> MAQALLVPPGPESFRLFTRESLAAIEKRAAEEKAKKPKKEQDNDDENKPKPNSDLEAGKNLPFIYGDIPPEMVSEPLEDLDPYYINKKTFIVMNKGKAIFRFSATSALYILTPLNPVRKIAIKILVHSLFSMLIMCTILTNCVFMTLSNPPDWTKNVEYTFTGIYTFESLIKILARGFCLEDFTFLRDPWNWLDFSVIVMAYVTEFVSLGNVSALRTFRVLRALKTISVIPGLKTIVGALIQSVKKLSDVMILTVFCLSVFALIGLQLFMGNLRNKCLQWPPSDSAFETNTTSYFNGTMDSNGTFVNVTMSTFNWKDYIGDDSHFYVLDGQKDPLLCGNGSDAGQCPEGYICVKAGRNPNYGYTSFDTFSWAFLSLFRLMTQDYWENLYQLTLRAAGKTYMIFFVLVIFLGSFYLVNLILAVVAMAYEEQNQATLEEAEQKEAEFQQMLEQLKKQQEEAQAVAAASAASRDFSGIGGLGELLESSSEASKLSSKSAKEWRNRRKKRRQREHLEGNNKGERDSFPKSESEDSVKRSSFLFSMDGNRLTSDKKFCSPHQSLLSIRGSLFSPRRNSKTSIFSFRGRAKDVGSENDFADDEHSTFEDSESRRDSLFVPHRHGERRNSNVSQASMSSRMVPGLPANGKMHSTVDCNGVVSLVGGPSALTSPTGQLPPEGTTTETEVRKRRLSSYQISMEMLEDSSGRQRAVSIASILTNTMEELEESRQKCPPCWYRFANVFLIWDCCDAWLKVKHLVNLIVMDPFVDLAITICIVLNTLFMAMEHYPMTEQFSSVLTVGNLVFTGIFTAEMVLKIIAMDPYYYFQEGWNIFDGIIVSLSLMELGLSNVEGLSVLRSFRLLRVFKLAKSWPTLNMLIKIIGNSVGALGNLTLVLAIIVFIFAVVGMQLFGKSYKECVCKINDDCTLPRWHMNDFFHSFLIVFRVLCGEWIETMWDCMEVAGQTMCLIVFMLVMVIGNLVVLNLFLALLLSSFSSDNLAATDDDNEMNNLQIAVGRMQKGIDYVKNKMRECFQKAFFRKPKVIEIHEGNKIDSCMSNNTGIEISKELNYLRDGNGTTSGVGTGSSVEKYVIDENDYMSFINNPSLTVTVPIAVGESDFENLNTEEFSSESELEESKEKLNATSSSEGSTVDVVLPREGEQAETEPEEDLKPEACFTEGCIKKFPFCQVSTEEGKGKIWWNLRKTCYSIVEHNWFETFIVFMILLSSGALAFEDIYIEQRKTIKTMLEYADKVFTYIFILEMLLKWVAYGFQTYFTNAWCWLDFLIVDVSLVSLVANALGYSELGAIKSLRTLRALRPLRALSRFEGMRVVVNALVGAIPSIMNVLLVCLIFWLIFSIMGVNLFAGKFYHCVNMTTGNMFDISDVNNLSDCQALGKQARWKNVKVNFDNVGAGYLALLQVATFKGWMDIMYAAVDSRDVKLQPVYEENLYMYLYFVIFIIFGSFFTLNLFIGVIIDNFNQQKKKFGGQDIFMTEEQKKYYNAMKKLGSKKPQKPIPRPANKFQGMVFDFVTRQVFDISIMILICLNMVTMMVETDDQGKYMTLVLSRINLVFIVLFTGEFV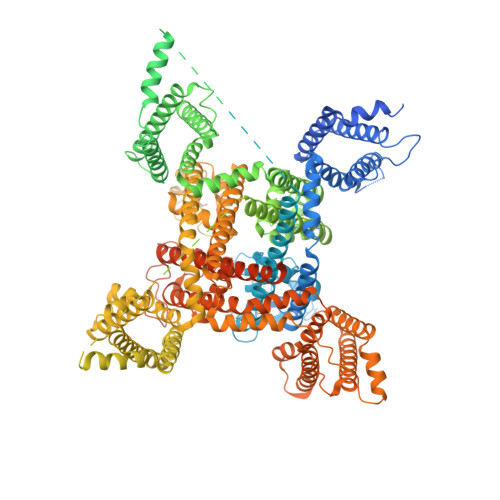LKLVSLRHYYFTIGWNIFDFVVVILSIVGMFLAEMIEKYFVSPTLFRVIRLARIGRILRLIKGAKGIRTLLFALMMSLPALFNIGLLLFLVMFIYAIFGMSNFAYVKKEAGIDDMFNFETFGNSMICLFQITTSAGWDGLLAPILNSAPPDCDPDTIHPGSSVKGDCGNPSVGIFFFVSYIIISFLVVVNMYIAVILENFSVATEESAEPLSEDDFEMFYEVWEKFDPDATQFIEFSKLSDFAAALDPPLLIAKPNKVQLIAMDLPMVSGDRIHCLDILFAFTKRVLGESGEMDALRIQMEDRFMASNPSKVSYEPITTTLKRKQEEVSAAIIQRNFRCYLLKQRLKNISSNYNKEAIKGRIDLPIKQDMIIDKLNG> MTNQKFFTLSNGNKIPAVAVVGTGTKWYKAEETDATFSQELTDIVKLSLDTVPGIVHIDAAETYKTYPELGAALKETKKPREEIFITDK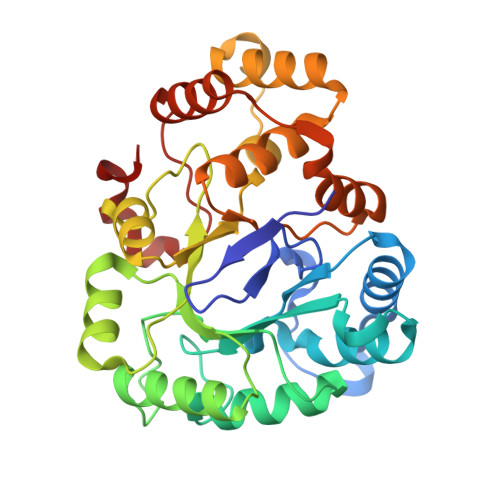FSSLHKISEDPKSALETALNKLGVDYVDLYLIHSPFFDKDLNIDLETAWKQLEELYKSGKAKNIGVSNFTVEDLKKVLAIAEIKPQVNQIEFSPFLQNQTPGIVEFSQKNDILLEAYSPLGPLQKKPTDADQQPFYQYLKELSEKYNKTEAQVLLLWVYKRGILPVTTSAKIERIKQAQDIFSFDLTEEEVKKITDLGLQHEPVRLWHVDFYTKYNSEAQK> GF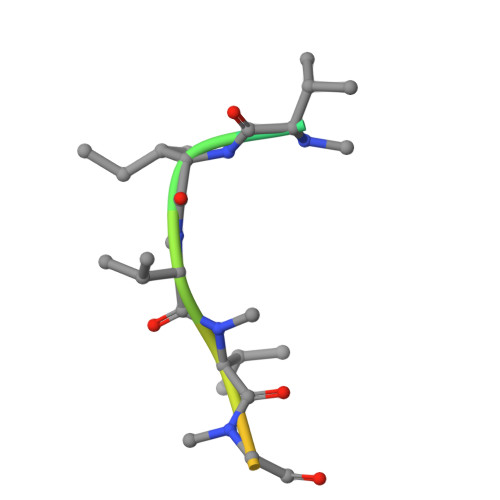PWVIVVGVIGVIG>GRPFVEMYSEIPEIIHMTEGRELVIPCRVTSPNITVTLKKFPLDTLIPDGKRIIWDSRKGFIISNATYKEIGLLTCEATVNGHLYKTNY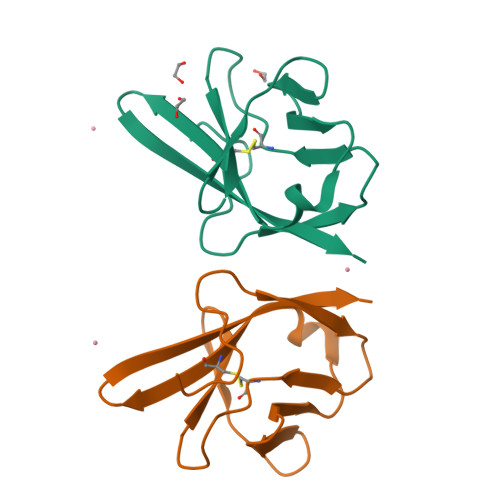LTHRQ[4x]>[6x]MKSSHHHHHHENLYFQSNYDWFSEMRKKDPVYYDGNIWQVFSYRYTKEVLNNFSKFSSDLTGYHERLEDLRNGKIRFDIPTRYTMLTSDPPLHDELRSMSADIF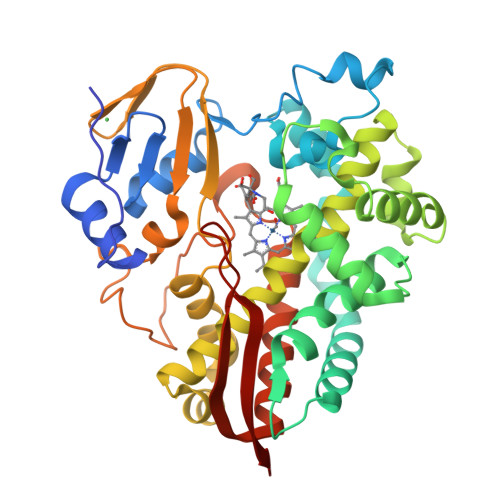SPQKLQTLETFIRETTRSLLDSIDPREDDIVKKLAVPLPIIVISKILGLPIEDKEKFKEWSDLVAFRWGKPGEIFELGKKYLELIGYVKDHLNSGTEVVSRVVNSNLSDIEKLGYIILLLIAGNEGTTNLISNSVIDFTRFNLWQRIREENLYLKAIEEALRYSPPLMRTVRKTKERVKLGDQTIEEGEYVRVWIASANRDEEVFHDGEKFIPDRNPNPHLSFGSGIHLGLGAPLARLEARIAIEEFSKRFRHIEILDTEKVPNEVLNGYKRLVVRLKSNE> NPWWAAFSRVCKDMNLTLEPEIMPAAGDNRYIRAVGVPALGFSPMNRTPVLLHDHDERLHEAVFLRGVDIYTRLLPAL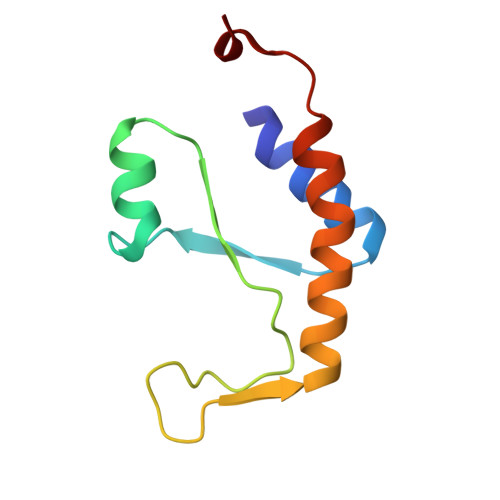ASVPALPSDS>[4x]ARSTNTFNYATYHTLDEIYDFMDLLVAQHPELVSKLQIGRSYEGRPIYVLKFSTGGSNRPAIWIDLGIHSREWITQATGVWFAKKFTENYGQNPSFTAILDSMDIFLEIVTNPNGFAFTHSENRLW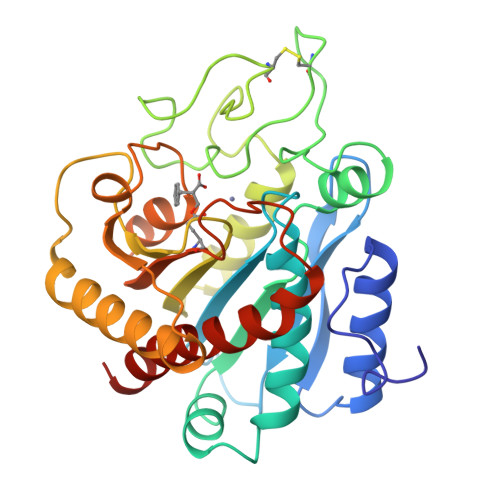RKTRSVTSSSLCVGVDANRNWDAGFGKAGASSSPCSETYHGKYANSEVEVKSIVDFVKNHGNFKAFLSIHSYSQLLLYPYGYTTQSIPDKTELNQVAKSAVAALKSLYGTSYKYGSIITTIYQASGGSIDWSYNQGIKYSFTFELRDTGRYGFLLPASQIIPTAQETWLGVLTIMEHTVNNLY> MNLEKLEVSHDADSLCVVIEISKHSNIKYELDKESGALMVDRVLYGAQNYPANYGFVPNTLGSDGDPVDALVL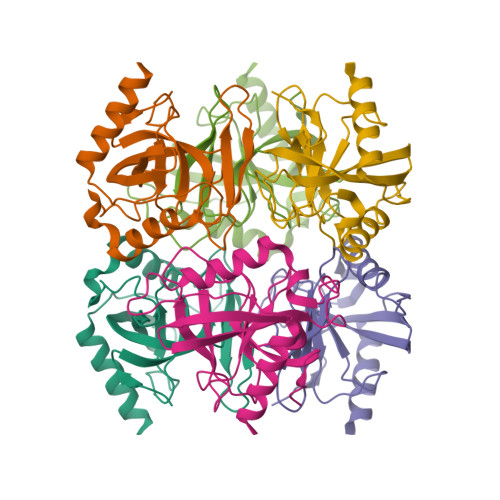SDVAFQAGSVVKARLVGVLNMEDESGMDEKLIALPIDKIDPTHSYVKDIDDLSKHTLDKIKHFFETYKDLEPNKWVKVKGFENKESAIKVLEKAIKAYQG> SWQTYVDTNLVGTGAVTQAAILGLDGNTWATSAGFAVTPAQGQTLASAFNNADPIRASGFDLAGVHYVTLRADDRSI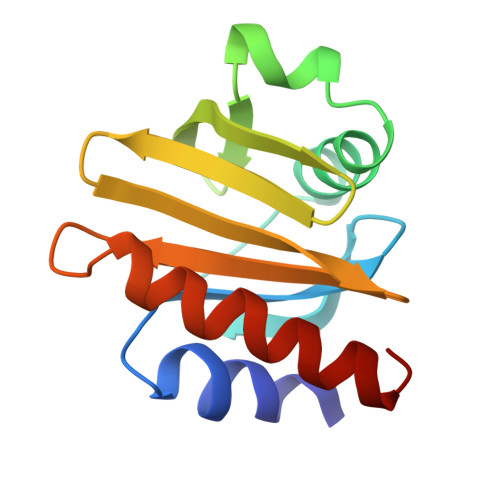YGKKGSAGVITVKTSKSILVGVYNEKIQPGTAANVVEKLADYLIGQGF> KQGPTSVAYVEVNNNSMLNVGKYTLADGGGNAFDVAVIFAANINYDTGTKTAYLHFNENVQRVLDNAVTQIRPLQQQGIKVLLSVLGNHQGAGFA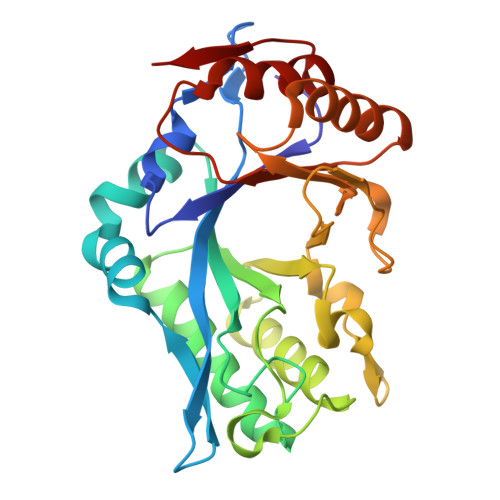NFPSQQAASAFAKQLSDAVAKYGLDGVDFNDQYAEYGNNGTAQPNDSSFVHLVTALRANMPDKIISLYNIGPAASRLSYGGVDVSDKFDYAWNPYYGTWQVPGIALPKAQLSPAAVEIGRTSRSTVADLARRTVDEGYGVYLTYNLDGGDRTADVSAFTRELYGSEAVRT>MAPKAKIVLVGSGMIGGVMATLIVQKNLGDVVLFDIVKNMPHGKALDTSHTNVMAYSNCKVSGSNTYDDLAGADVVIVTAGFTKAPGKSDKEWNRDDLLPLNNKIMIEIGGHIKKNCPNAFIIVVTNPVDVMVQLLHQHSGVPKNKIIGLGGVLDTSRLKYYISQKLNVCPRDVNAHIVGAHGNKMVLLKRYITVGGIPLQEFINNKLISDAELEAIFDRTVNTALEIVNLHASPYVAPAAAIIEMAESYLKDLKKVLICSTLLEGQYGHSDIFGGTPVVLGANGV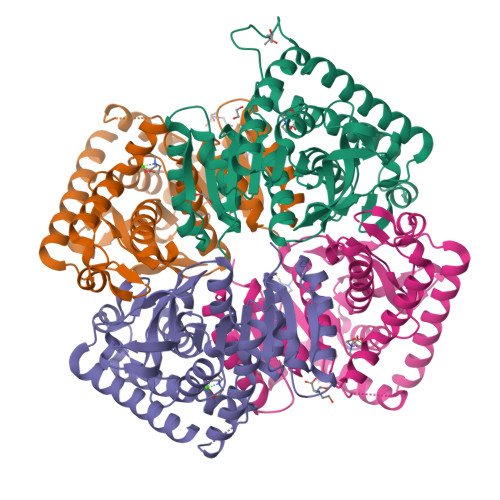EQVIELQLNSEEKAKFDEAIAETKRMKALAHHHHHH[4x]Plicamycin, mithramycin analogue 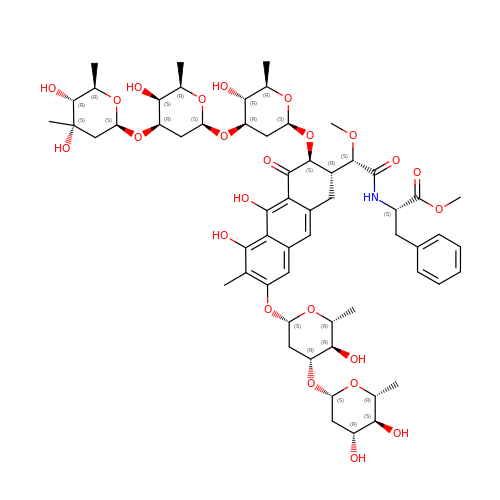MTM SA-Phe | C59 H81 N O24 | WHRHJGQUYQCUGP-NIMSAUJISA-N>FTLIELMIVVAIIGILAAIAIPQYQNYVARSEGASALATINPLKTTVEESLSRGIAGSKIKIGTTASTATETYVGVEPDANKLGVIAVAIEDSGAGDITFTFQTGTSSPKNATKVITLNRTADGVWACKSTQDPMFTPKGCDN[23x]

Type IV pili (T4Ps) are abundant in many bacterial and archaeal species, where they play important roles in both surface sensing and twitching motility, with implications for adhesion, biofilm formation and pathogenicity. Bacterial surface pili are assembled by repeated interactions of monomeric protein subunits called pilins, leading to the formation of a filamentous structure that protrudes from the cell and binds to surfaces. As P. aeruginosa T4Ps mediate surface sensing, the first step of biofilm formation, they play a key role in allowing P. aeruginosa to transition from a unicellular planktonic to a multicellular biofilm state. PilA subunits constituting the T4P exhibit a classical pilin fold featuring an extended N-terminal α-helix linked to a C-terminal globular β-sheet-containing domain, which are packed tightly along the pilus, in line with models derived from previous cryo-EM data of the P. aeruginosa PAK strain.

In this study, we describe a 3.2 Å-resolution cryo-EM structure of the fully assembled P. aeruginosa T4P from the model PAO1 strain, the highest-resolution structure of a P. aeruginosa T4P using cryo-EM to date. To study the structure of the P. aeruginosa T4P, we used a PAO1 strain with a deletion of the retraction ATPase pilT to maximise pilus decoration on the cell surface. The atomic model confirms a tubular arrangement of the P. aeruginosa PAO1 T4P, with a helical rise of 10.17 Å and a right-handed twist of 87.4° per subunit, resulting in an overall helical pitch of 41.9 Å. The innermost part of the T4P is stabilised by hydrophobic interactions of the N-terminal α-helices of PilA, which contain a row of hydrophobic residues (amino acid residues 1–16, where residue 1 is the N-terminus of the mature pilin), forming the core of the T4P in a staggered arrangement. These N-terminal helices in turn interact with the helices of the globular domain through further hydrophobic interactions. Moreover, ionic interactions and hydrogen bonds, mainly involving the loops in the pilin globular domains, stabilise the interfaces among multiple pilin subunits along the assembled pilus. For example, the Q23 and Q25 residues of every pilin subunit N interact with the β3-β4-loop of subunit N-4 and the αβ-loop of subunit N-3. Similarly, residue K139 of every subunit N interacts with the β2-β3-loop of subunit N+1 and the αβ-loop of subunit N-3. In addition, the C-terminal region of the P. aeruginosa PilA contains two buried cysteine residues (C128, C141) in close proximity, which form a disulfide bond resolved in our map, constituting a structural feature present in many known T4P structures. P. aeruginosa PAO1, however, is a strain that encodes a Group 2 pilin that is not glycosylated, in good agreement with our cryo-EM density which did not show any densities that are not accounted for by the polypeptide chain itself.>MANKPTQPLFPMGLETSESSNIKGFNNSGTMEHSPGAVMTFPEDTEVTGLPSSVRYNPDSDEFEGYYENGGWLSLGGGGIRWETLPHAPSSNLLEGRGYLINNTTGTSTVVLPSPTRIGDSVTICDAYGKFATYPLTVSPSGNNMYGSTEDMAITTDNVSATFTWSGPEQGWVITSGVGLGQGRVYSREIFTQILASETSAVTLNTPPTIVDVYADGKRLAESKYSLDGNVITFSPSLPASTELQVIEYTPIQLGNGGGSGSSTITWVYNGGSAIGGETEITLDIVVDDVPAIDINGSRQYKNLGFTFDPLTSKITLAQELDAEDEVVVIINGTPHHHHH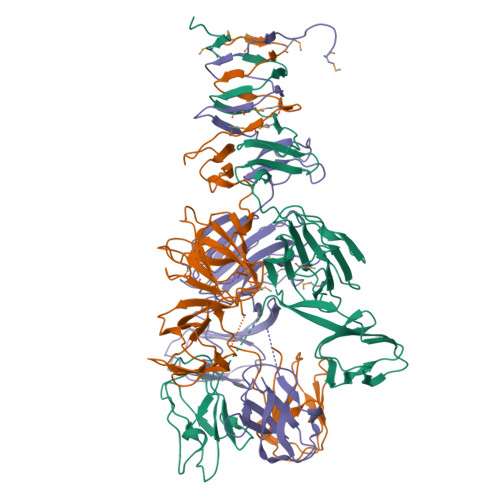H[3x]[3-{4-[6-(1-methyl-1H-pyrazol-4-yl)pyrazolo[1,5-a]pyrazin-4-yl]-1H-pyrazol-1-yl}-1-(2,2,2-trifluoroethyl)azetidin-3-yl]acetonitrile 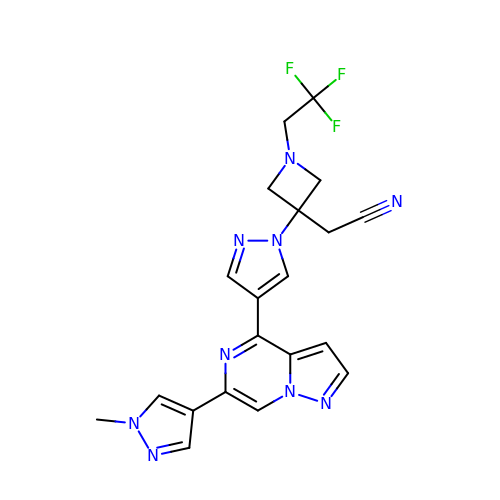| C20 H18 F3 N9 | CVWIGSVNTPFWIS-UHFFFAOYSA-N> LYFQGMEERSQLFLEQYLSSVSREVSEKYTSFSADYFCADEYNANVCADL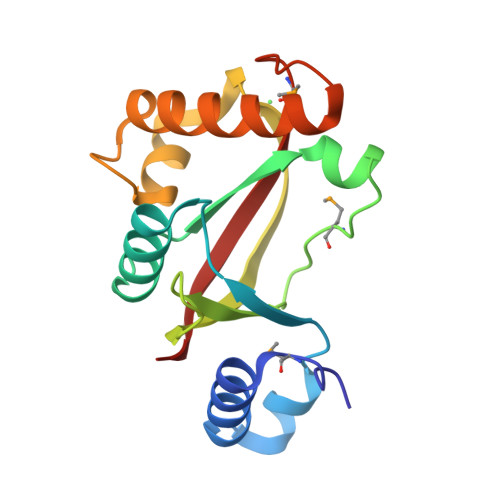ILRGEKRASCSLEYWYSQKGELMPQVGHLQVVTNWDGKPICIIEITSVSKCQYNQVSEDFAASEGEGDKSLAWWQEAHRNFFSRECHELGIEFREDMLLVLEHFKVVYH2-(4-((9S,10S,14S,Z)-18-(2-AMINO-2-OXOETHYL)-9-(CARBOXYMETHYL)-14-(NAPHTHALEN-1-YLMETHYL)-8,17,20-TRIOXO-7,16,19-TRIAZASPIRO[5.14]ICOS-11-EN-10-YL)PHENYL)MALONIC 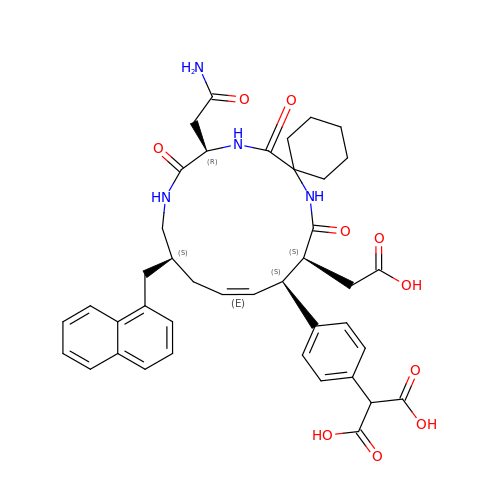ACID | C41 H46 N4 O10 | FYIJOFSDJMOTGX-HGOOHLDYSA-N>[4x]HHHHHHTDVVIVSAARTAVGKFGGSLAKIPAPELGAVVIKAALERAGVKPEQVSEVIMGQVLTAGSGQNPARQAAIKAGLPAMVPAMTINKVSGSGLKAVMLAANAIMAGDAEIVVAGGQENMSAAPHVLPGSRDGFRMGDAKLVD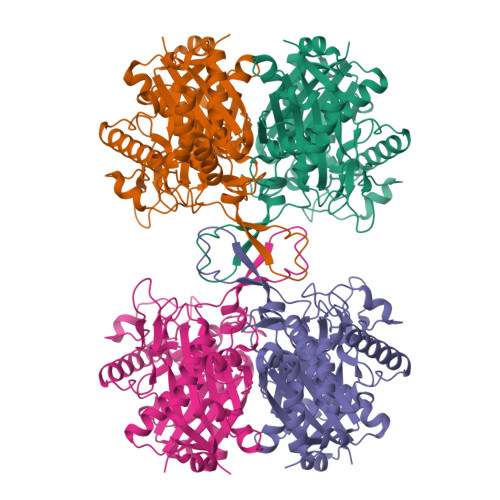TMIVDGLWDVYNQYHMGITAENVAKEYGITREAQDEFAVGSQNKAEAAQKAGKFDEEIVPVLIPQRKGDPVAFKTDEFVRQGATLDSMSGLKPAFDKAGTVTAANASGLNDGAAAVVVMSAAKAKELGLTPLATIKSYANAGVDPKVMGMGPVPASKRALSRAEWTPQDLDLMEINEAFAAQALAVHQQMGWDTSKVNVNGGAIAIGHPIGASGCRILVTLLHEMKRRDAKKGLASLCIGGGMGVALAVERK> MRRNRRGSPARPAARFVRPAIPSALSVALLVCTPGLATADPQTDTIAALIADVAKANQRLQDLSDEVQAEQESVNKAMVDVETARDNAAAAEDDLEVSQRAVKDANAAIAAAQHRFDTFAAATYMNGPSVSYLSASSPDEIIATVTAAKTLSASSQAVMANLQRARTERVNTES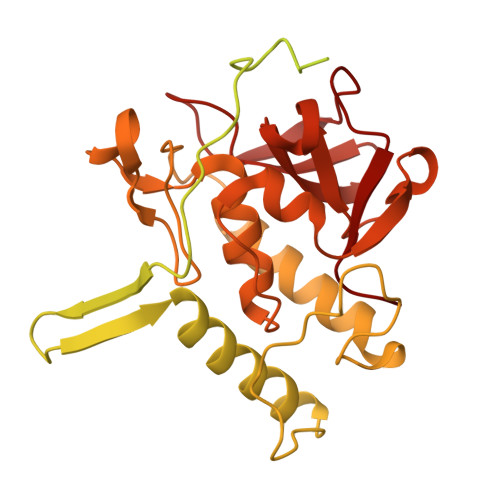AARLAKQKADKAAADAKASQDAAVAALTETRRKFDEQREEVQRLAAERDAAQARLQAARLVAWSSEGGQGAPPFRMWDPGSGPAGGRAWDGLWDPTLPMIPSANIPGDPIAVVNQVLGISATSAQVTANMGRKFLEQLGILQPTDTGITNAPAGSAQGRIPRVYGRQASEYVIRRGMSQIGVPYSWGGGNAAGPSKGIDSGAGTVGFDASGLVLYSFAGVGIKLPHYSGSQYNLGRKIPSSQMRRGDVIFYGPNGSQHVTIYLGNGQMLEAPDVGLKVRVAPVRTAGMTPYVVRYIEY> AVCGSVWGQ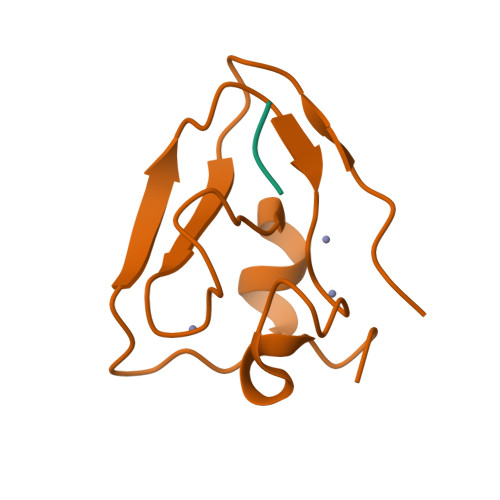NDLAYRCRTCEHDPTCAICVPCFQNGNHKDHDYSIMYTGGGCCDCGDTTAWKREGFCSRHKGA;> RDG>[2x]GSTLQPLENSTRQEKLLYPKLNQLSNSINAAVAFLL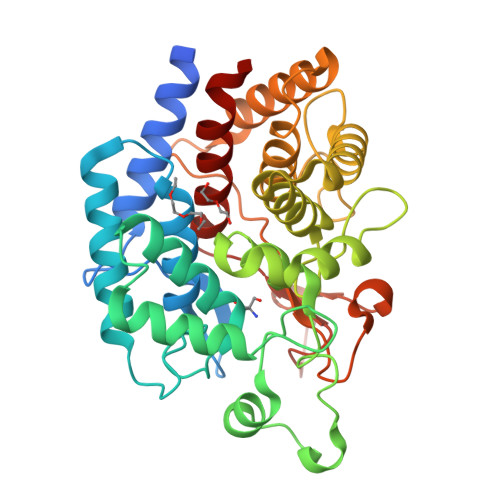EARNLEGWWQDFNFPQAASIGDEWVTAYVGTMLATLPYAHVHEALMQAWELLKIRDHRPTGEWGYNYILCGDADTTGWALQLAAAVGASDSERAQQARAALATHLQPNGGIATFAEESIRAYIKVPDLANVSFQGWCGAHTCVSAAVAALPEFRSRLHDYLRVTQTSQGNWEGYWWSDHEYTTALTAEALAAGGQAADQPSIEQAVAWGLKRLCPQGFVATSKHPNGSTFATAWCLRLLLLNTVDAEVKAARAAAIGWLLEQQRPNGSWVSSAYLRIPYPFDRNPNQFPHWRYYDEIEGDKRFEGSIIFDHNSIFTTATVVNSLVKAAPML>[2x]GLKEH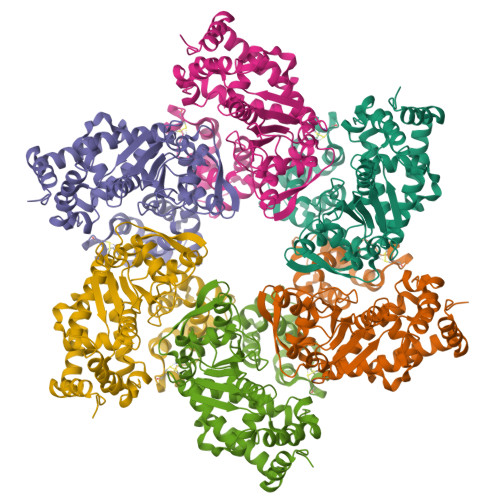DFNPEEAEETKQVSWKLVTEYAMETKCDDVLLLLGMYLEFQYSFEMCLKCIKKEQPSHYKYHEKHYANAAIFADSKNQKTICQQAVDTVLAKKRVDSLQLTREQMLTNRFNDLLDRMDIMFGSTGSADIEEWMAGVAWLHCLLPKMDSVVYDFLKCMVYNIPKKRYWLFKGPIDSGKTTLAAALLELCGGKALNVNLPLDRLNFELGVAIDQFLVVFEDVKGTGGESRDLPSGQGINNLDNLRDYLDGSVKVNLEKKHLNKRTQIFPPGIVTMNEYSVPKTLQARFVKQIDFRPKDYLKHCLERSEFLLEKRIIQSGIALLLMLIWYRPVAEFAQSIQSRIVEWKERLDKEFSLSVYQKMKFNVAMGIGVLD>MSEMSSFLHIGDIVSLYAEGSVNGFISTLGLVDDRCVVEPAAGDLDNPPKKFRDCLFKVCPMNRYSAQKQYWKAKQTKQDKEKIADVVLLQKLQHAAQMEQKQNDTENKKVHGDVVKYGSVIQLLHMKSNKYLTVNKRLPALLEKNAMRVTLDATGNEGSWLFIQPFWKLRSNGDNVVVGDKVILNPVNAGQPLHASNYELSDNAGCKEVNSVNCNTSWKINLFMQFRDHLEEVLKGGDVVRLFHAEQEKFLTCDEYKGKLQVFLRTTLRQSATSATSSNALWEVEVVHHDPCRGGAGHWNGLYRFKHLATGNYLAAEENPSYKGDASDPKAAGMGAQGRTGRRNAGEKIKYCLVAVPHGNDIASLFELDPTTLQKTDSFVPRNSYVRLRHLCTNTWIQSTNVPIDIEEERPIRLMLGTCPTKEDKEAFAIVSVPVSEIRDLDFANDASSMLASAVEKLNEGFISQNDRRFVIQLLEDLVFFVSDVPNNGQNVLDIMVTKPNRERQKLMREQNILKQVFGILKAPFREKGGEGPLVRLEELSDQKNAPYQHMFRLCYRVLRHSQEDYRKNQEHIAKQFGMMQSQIGYDILAEDTITALLHNNRKLLEKHITKTEVETFVSLVRKNREPRFLDYLSDLCVSNHIAIPVTQELICKCVLDPKNSDILIRTELRPVKEMAQSHEYLSIEYSEEEVWLTWTDKNNEHHEKSVRQLAQEARAGNAHDENVLSYYRYQLKLFARMCLDRQYLAIDEISQQLGVDLIFLCMADEMLPFDLRASFCHLMLHVHVDRDPQELVTPVKFARLWTEIPTAITIKDYDSNLNASRDDKKNKFANTMEFVEDYLNNVVSEAVPFANEEKNKLTFEVVSLAHNLIYFGFYSFSELLRLTRTLLGIIDCVQGPPAMLQAYEDPGGKNVRRSIQGVGHMMSTMVLSRKQSVFSAPSLSAGASAAEPLDRSKFEENEDIVVMETKLKILEILQFILNVRLDYRISYLLSVFKKEFVEVFPMQDSGADGTAPAFDSTTANMNLDRIGEQAEAMFGVGKTSSMLEVDDEGGRMFLRVLIHLTMHDYAPLVSGALQLLFKHFSQRQEAMHTFKQVQLLISAQDVENYKVIKSELDRLRTMVEKSELWVDKKGSGKGEEVEAGAAKDKKERPTDEEGFLHPPGEKSSENYQIVKGILERLNKMCGVGEQMRKKQQRLLKNMDAHKVMLDLLQIPYDKGDAKMMEILRYTHQFLQKFCAGNPGNQALLHKHLHLFLTPGLLEAETMQHIFLNNYQLCSEISEPVLQHFVHLLATHGRHVQYLDFLHTVIKAEGKYVKKCQDMIMTELTNAGDDVVVFYNDKASLAHLLDMMKAARDGVEDHSPLMYHISLVDLLAACAEGKNVYTEIKCTSLLPLEDVVSVVTHEDCITEVKMAYVNFVNHCYVDTEVEMKEIYTSNHIWTLFENFTLDMARVCSKREKRVADPTLEKYVLSVVLDTINAFFSSPFSENSTSLQTHQTIVVQLLQSTTRLLECPWLQQQHKGSVEACIRTLAMVAKGRAILLPMDLDAHISSMLSSGASCAAAAQRNASSYKATTRAFPRVTPTANQWDYKNIIEKLQDIITALEERLKPLVQAELSVLVDVLHWPELLFLEGSEAYQRCESGGFLSKLIQHTKDLMESEEKLCIKVLRTLQQMLLKKTKYGDRGNQLRKMLLQNYLQNRKSTSRGDLPDPIGTGLDPDWSAIAATQCRLDKEGATKLVCDLITSTKNEKIFQESIGLAIHLLDGGNTEIQKSFHNLMMSDKKSERFFKVLHDRMKRAQQETKSTVAVNMNDLGSQPHEDREPVDPTTKGRVASFSIPGSSSRYSLGPSLRRGHEVSERVQSSEMGTSVLIMQPILRFLQLLCENHNRDLQNFLRCQNNKTNYNLVCETLQFLDIMCGSTTGGLGLLGLYINEDNVGLVIQTLETLTEYCQGPCHENQTCIVTHESNGIDIITALILNDISPLCKYRMDLVLQLKDNASKLLLALMESRHDSENAERILISLRPQELVDVIKKAYLQEEERENSEVSPREVGHNIYILALQLSRHNKQLQHLLKPVKRIQEEEAEGISSMLSLNNKQLSQMLKSSAPAQEEEEDPLAYYENHTSQIEIVRQDRSMEQIVFPVPGICQFLTEETKHRLFTTTEQDEQGSKVSDFFDQSSFLHNEMEWQRKLRSMPLIYWFSRRMTLWGSISFNLAVFINIIIAFFYPYMEGASTGVLDSPLISLLFWILICFSIAALFTKRYSIRPLIVALILRSIYYLGIGPTLNILGALNLTNKIVFVVSFVGNRGTFIRGYKAMVMDMEFLYHVGYILTSVLGLFAHELFYSILLFDLIYREETLFNVIKSVTRNGRSILLTALLALILVYLFSIVGFLFLKDDFILEVDRLPNNHSTASPLGMPHGAAAFVDTCSGDKMDCVSGLSVPEVLEEDRELDSTERACDTLLMCIVTVMNHGLRNGGGVGDILRKPSKDESLFPARVVYDLLFFFIVIIIVLNLIFGVIIDTFADLRSEKQKKEEILKTTCFICGLERDKFDNKTVSFEEHIKLEHNMWNYLYFIVLVRVKNKTDYTGPESYVAQMIKNKNLDWFPRMRAMSLVXXXXXXXXXXXXXXXXXXXXXX[4x]

A pivotal component of the calcium (Ca2+) signaling toolbox in cells is the inositol 1,4,5-triphosphate (IP3) receptor (IP3R), which mediates Ca2+ release from the endoplasmic reticulum (ER), controlling cytoplasmic and organellar Ca2+ concentrations. IP3Rs are co-activated by IP3 and Ca2+, inhibited by Ca2+ at high concentrations, and potentiated by ATP. There are three IP3R subtypes (IP3R-1, -2, and -3) that share 60–70% sequence identity, form homo- or hetero-tetramers, exhibit different spatial expression profiles, and are involved in different signaling pathways. Each IP3R subunit is about 2700 amino acids in length and contains a transmembrane domain (TMD) and a large cytoplasmic region comprising two β-trefold domains (βTF1 and βTF2), three Armadillo repeat domains (ARM1, ARM2, and ARM3), a central linker domain (CLD), a juxtamembrane domain (JD), and a short C-terminal domain (CTD)6–10. Here we report cryo-electron microscopy (cryo-EM) structures of human type-3 IP3R obtained from a single dataset in multiple gating conformations: IP3-ATP bound pre-active states with closed channels, IP3-ATP-Ca2+ bound active state with an open channel, and IP3-ATP-Ca2+ bound inactive state with a closed channel.

Three structures have closed pores with well-resolved densities for IP3 and ATP and are referred to as pre-active A, B, and C. The pre-active B and C structures adopt distinct conformations that are intermediates between the pre-active A and open state structures. Based on these conformational changes, we propose a sequential transition from pre-active A to B, then C, although the alternative transitions cannot be ruled out entirely. Within the JD, we observed a well-resolved cryo-EM density for ATP in all the structures. The adenosine base intercalates into a cavity surrounded by F2156, F2539, I2559, M2565, and W2566 near the zinc finger motif and forms hydrogen bonds with the sulfur of C2538, the backbone amide group of F2539, and the carbonyl groups of H2563 and I2559. The phosphate moieties interact with K2152, K2560, and N2564. There are no apparent structural changes around the binding site upon ATP binding, suggesting that ATP’s potentiating effect is likely due to the increased rigidity of the JD. In the closed channel, F2513 and I2517 of the S6 helix form two layers of hydrophobic constriction at the pore, blocking the path for the permeation of hydrated ions. Our structures reveal that IP3 binding leads to several conformational changes at the NTD, ARM3, and JD, without any apparent structural changes at the activatory Ca2+ binding site, and that the ARM3 and JD adopt a new pre-gating conformation relative to the TMD with modest changes at the intersubunit interface between the JDs at the cytoplasmic side of the TMD.>MASHDKQFSLFLHKASAHGWKVAFVLEELSLSYEIVLVDVAKNEQKSPEFMKLNPNGRTPALIDHGNSDFVIWESNAMVQYVADKYDTERKISMAPGTDDFYIQLQWQYFQGTGQGPYFGQLVWFTLYHEEKIPSAVTRYKEEALRVFSVLERVLSNQEWLV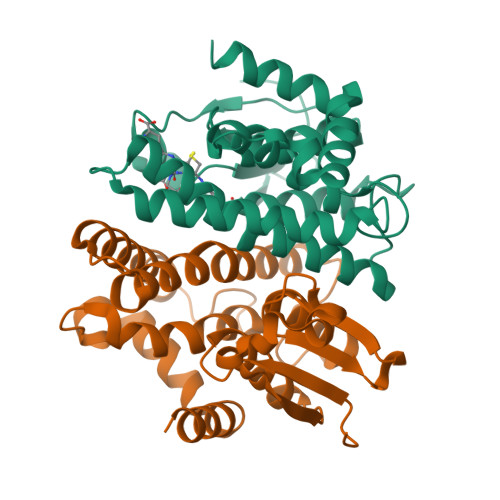GGKMTIADISFVSWNDMIVHFLDNFDFEKEFPATAAWHYKMLKRPTIKRPWDERRKLMSRQ[4x]> MGCTLSAEDKAAVERSKMIDRNLREDGERSARLVKILLLGAGESGKSTFLKQMRIIHGQDFDQRAREEFRPTIYSNVIKGMRVLVDAREKLHIPWGDNKNQLHGDKLMAFDTRAPMAAQGMVETRVFLQYLPAIRALWEDSGIQNAYDRRREFQLGESVKYFLDNLDKLGVPDYIPSQQDILLARRPTKGIHEYDFEIKNVPFKMVDVGGQRSERKRWFECFDSVTSILFLVSSSEFDQVLMEDRQTNRLTESLNIFETIVNNR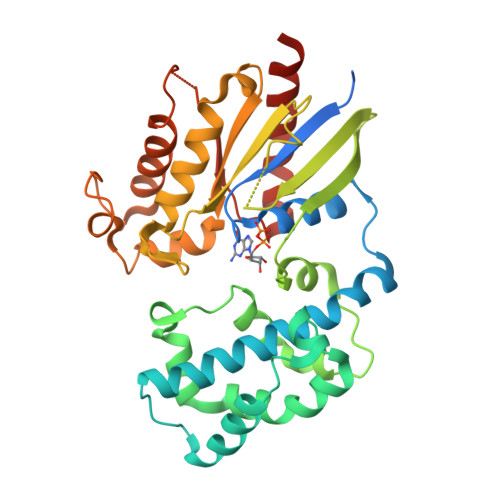VFSNVSIILFLNKTDLLEEKVQVVSIKDYFLEFEGDPHCLRDVQKFLVECFRGKRRDQQQRPLYHHFTTAINTENIRLVFRDVKDTILHDNLKQLMLQ> QTSVSPSKVILPRGGSVLVTCSTSCDQPKLLGIETPLPKKELLLPGNNRKVYELSNVQEDSQPMCYSNCPDGQSTAKTFLTVYWTPERVELAPLPSWQPVGKNLTLRCQVEGGAPRANLTVVLLRGEKELKREPAVGEPAEVTTTVLVRRDHHGANFSCR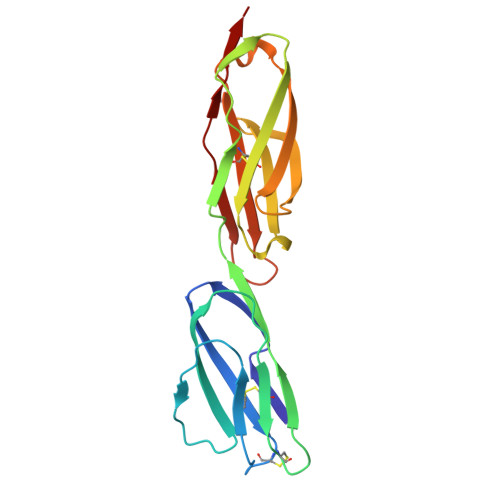TELDLRPQGLELFENTSAPYQLQTFG>MSFINYSSREINCKIVYYGPGLCGKTTNLQYIYNKTAAETKGKLISLSTETDRTLFFDFLPLSLGEIRGFKTRFHLYTVPGQVFYDASRKLILKGVDGVVFVADSQIERMEANMESLENLRINLAEQGYDLNKIPYVIQYNKRDLPNAVTVEEMRKA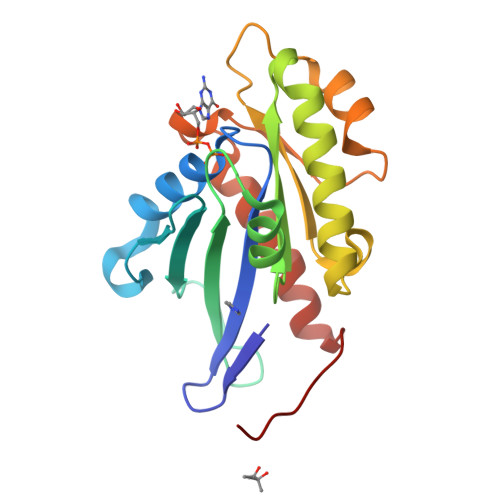LNHRNIPEYQAVAPTGVGVFDTLKAVAKLVLTELKKGGGSHHHHHH[2x]>GGSMNKLYIGNLSENAAPSDLE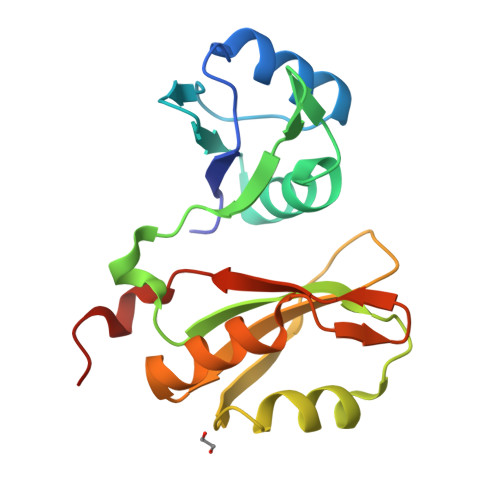SIFKDAKIPVSGPFLVKTGYAFVDCPDESWALKAIEALSGKIELHGKPIEVEHSVPKRQRIRKLQIRNIPPHLQWEVLDSLLVQYGVVESCEQVNTDSETAVVNVTYSSKDQARQALDKLNGFQLENFTLKVAYIPDEMAAQHHHHHH[2x]> MKELIVYFSTQSNNTHRFVQKLDAESIRIPIDEEERIKVDEDYVLIVPTYSGGKVTDAGQVDAHGAVPKQVIHFLNDPDNRKHCLGVISSGNTNFGDSFAIAGPVISYKLKVPLLYQFELIGTKEDVEEVNRIISETFNAD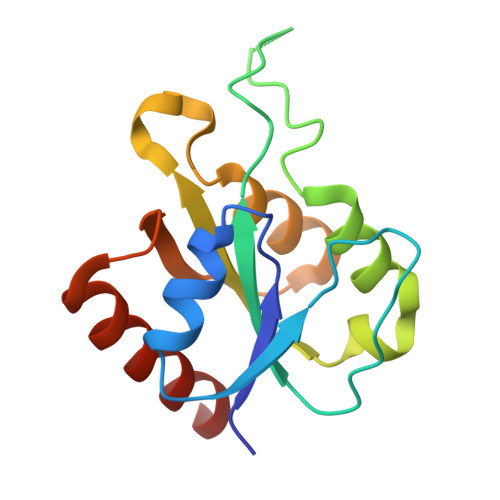Q> ETPPRFTRTPVDQTGVSGGVASFICQATGDPRPKIVWNKKGKKVSNQRFEVIEFDDGSGSVLRIQPLRTPRDEAIYECVASNNVGEISVSTRLTVLRED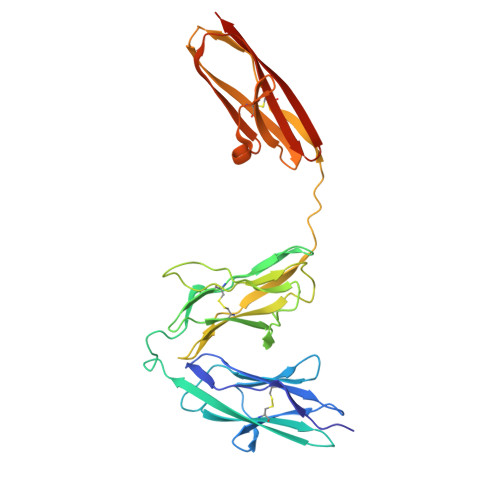QIPRGFPTIDMGPQLKVVERTRTATMLCAASGNPDPEITWFKDFLPVDTSNNNGRIKQLRSESIGGTPIRGALQIEQSEESDQGKYECVATNSAGTRYSAPANLYVRELREVRRVPPRFSIPPTNHEIMPGGSVNITCVAVGSPMPYVKWMLGAEDLTPEDDMPIGRNVLELNDVRQSANYTCVAMSTLGVIEAIAQITVKALSRLVPR> HHHHHHSQDPMNALTTIDFNQHVIVRLPSKNYKIVELKPNTSVSLGKFGAFEVNDIIGYPFGLTFEIYYDGEEVSSDENRDSKPKNKIPIGKVRLLSQEIKDVNNDKDDGQSEPPLSIKEKSVSLELSSIDSSATNQNLVNMGSKAQELTVEEIEKMKQESLSSKEIIDKIIKSHKSFHNKTVYSQEKYVNRKKQKFAKYFTVEYLSSSNLLQFLIDKGDIQRVLDMSQESMGMLLNLANIQSEGNYLCMDETGGLLVYFLLERMFGGDNESKSKGKVIVIHENEHANLDLLKFANYSEKFIKEHVHTISLLDFFEPPTLQEIQSRFTPLPKEEARALKGGKKNSYYRKLRWYNTQWQILELTGEFLYDGLVMATTLHLPTLVPKLAEKIHGSRPIVCYGQFKETLLELAHTLYSDLRFLAPSILETRCRPYQSIRGKLHPLMTMKGGGGYLMWCHRVIPAPEPVSENATAADSSEKLAEHGAKKQKI;> MSTNCFSGYKDLIKEGDLTLIWVSRDNIKPVRMHSEEVFNTRYGSFPHKDIIGKPYGSQIAIRTKGSNKFAFVHVLQPTPELWTLSLPHRTQIVYTPDSSYIMQRLNCSPHSRVIEAGTGSGSFSHAFARSVGHLFSFEFHHIRYEQALEEFKEHGLIDDNVTITHRDVCQGGFLIKKGDTTSYEFGNNETAASLNANVVFLDLPAPWDAIPHLDSVISV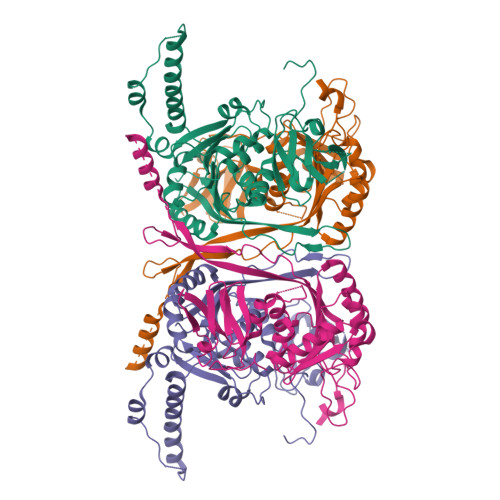DEKVGLCCFSPCIEQVDKTLDVLEKYGWTDVEMVEIQGRQYESRRQMVRSLNDALERLRDIKRHKLQGVERRKRMFNNTIDSNDEKVGKRNEDGVPLTEKAKFNPFGKGSRIKEGDSNYKWKEVTKMEAEIKSHTSYLTFAFKVVNRSRDDEKVNEILRSTEK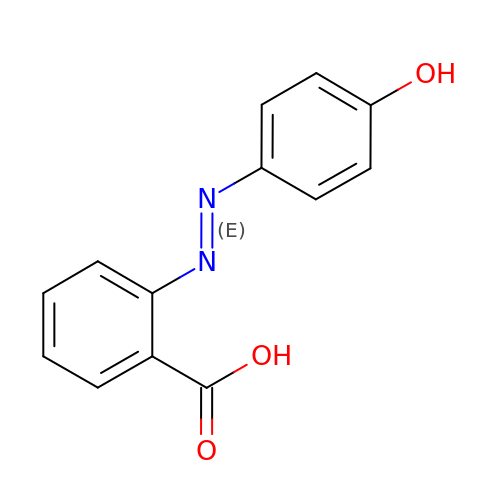2-((4'-HYDROXYPHENYL)-AZO)BENZOIC ACID | C13 H10 N2 O3 | DWQOTEPNRWVUDA-CCEZHUSRSA-N>MKTFAAYVIIACLSSTALAGSITENMSWNKEFSAEAVNGVFVLCKSSS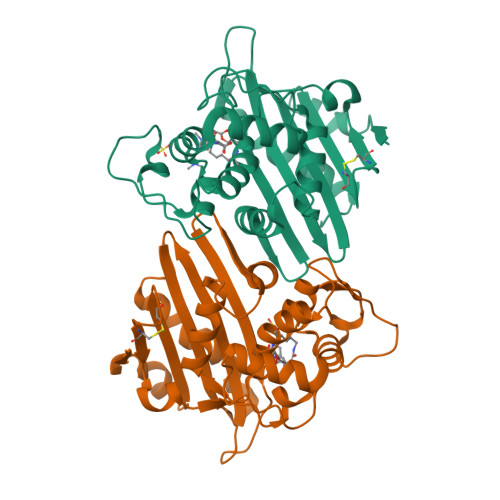KSCATNDLARASKEYLPASTFKIPNAIIGLETGVIKNEHQVFKWDGKPRAMKQWERDLTLRGAIQVSALPVFQQIAREVGEVRMQKYLKKFSYGNQNISGGIDKFWLEGQLRISAVNQVEFLESLYLNKLSASKENQLIVKEALVTEAAPEYLVHSKTGFSGVGTESNPGVAWWVGWVEKETEVYFFAFNMDIDNESKLPLRKSIPTKIMESEGIIGG[4x]> GSHMDSYELSPQLEELITKVSKAHQETFPSLCQLGKYTTNSSADHRVQLDLGLWDKFSELATKCIIKIVEFAKRLPGFTGLSIADQITLLKAACLDILMLRIC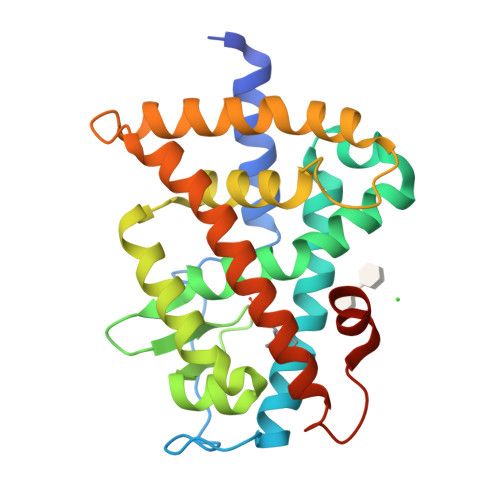TRYTPEQDTMTFSDGLTLNRTQMHNAGFGPLTDLVFAFAGQLLPLEMDDTETGLLSAICLICGDRMDLEEPEKVDKLQEPLLEALRLYARRRRPEQPYMFPRMLMKITDLRGISTKGAERAITLKMEIPGPMPPLIREMLENPEMFE>[2x]MKILVTNDDGVHSPGLRLLYQFALSLGDVDVVAPESPKSATGLGITLHKPLRMYEVDLCGFRAIATSGTPSDTVYLATFGLGRKYDIVLSGINLGDNTSLQVILSSGTL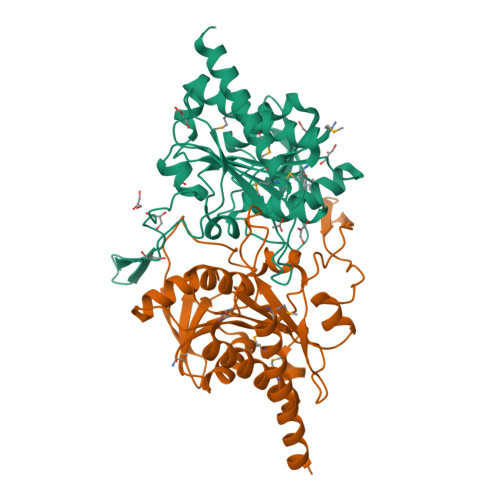GAAFQAALLGIPALAYSAYLENWNELLNNKEAVEIMGAVVSSTASYVLKNGMPQGVDVISVNFPRRLGRGVRAKLVKAAKLRYAQQVVERVDPRGVRYYWLYGRDLAPEPETDVYVVLKEGGIAITPLTLNLNAVDAHREVDMDSLNRMVEYINASLSKLAAALEHHHHHH>MGSSHHHHHHSQDPNSMSQPFASRGLAWFQALAGSLAPRPGDPASLRVADAELDGYPVRFLAVVPDPDNPFPRARQGEVGLLEGWGLAAAVDEALEADREAPRKRALLAIVDVPSQAYGRREEALGIHQALAGAVDAYARARLAGHPLIGLLVGKAMSGAFLAHGYQANRLIALHDPGVMVHAMGKAAAARITLRSVEELEALAAKVPPMAYDIDSYASLGLLWRTLPVETVEVPSTADLVRVRTCLGEALADILGGPRDLGGRLGAANREASARVRRLLREQW[2x];>MTDVARLLALRSFTELGARQRARALLDAGSFRELLDPFAGVQSPWLERQGIVPQADDGVVVARGLLDGQPAVLAAIEGAFQGGSLGEVSGAKIAGALELAAEDNRNGVPTRALLLLETGGVRLQEANLGLAAIAEIQAAIVDLQRYQPVVAVIAGPVGCFGGMSIAAGLCSYVLVTREARLGLNGPQVIEQEAGIAEYDSR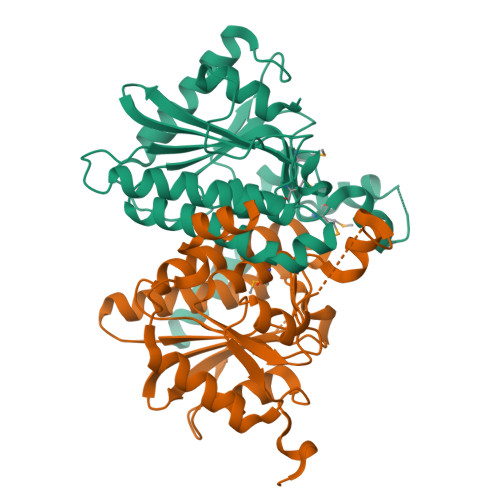DRPFIWSLTGGEQRFASGLADAYLADDLDEVRTSVLAYFAKGLPARPRCRRAEDYLRRLGDLDTAEQPDAAGVRRLYQGLGQGDAT[2x]>[5x]MSNFKVRDPVIQERLDHDYAHHPLVARMNTLDQGNMSQAEYLVQKRHYLVFLIAHHYYEAYLRRMGGIQRRDHLQTLRDQKPRERADRVSAASAYDAGTFTVPSRPGPASGTTPGGQDSLGVSGSSITTLSSGPHSLSPASDILTTLSSTTETAAPAVADARKPPSGKKK;>[5x]MEATLEQRPFPYLATEANLLTQIKESAADGLFKSFQLLLGKDAREGSVRFEALLGVYTNVVEFVKFLETALAAACVNTEFKDLRRMIDGKIQFKISMPTIAHGDGRRPNKQRQYIVMKACNKHHIGAEIELAAADIELLFAEKETPLDFTEYAGAIKTITSALQFGMDALERGLVDTVLAVKLRHAPPVFILKTLGDPVYSERGLKKAVKSDMVSMFKAHLIEHSFFLDKAELMTRGKQYVLTMLSDMLAAVCEDTVFKGVSTYTTASGQQVAGVLETTDSVMRRLMNLLGQVESAMSGPAAYASYVVRGANLVTAVSYGRAMRNFEQFMARIVDHPNALPSVEGDKAALADGHDEIQRTRIAASLVKIGDKFVAIESLQRMYNETQFPCPLNRRIQYTYFFPVGLHLPVPRYSTSVSVRGVESPAIQSTETWVVNKNNVPLCFGYQNALKSICHPRMHNPTQSAQALNQAFPDPDGGHGYGLRYEQTPNMNLFRTFHQYYMGKNVAFVPDVAQKALVTTEDLLHPTSHRLLRLEVHPFFDFFVHPCPGARGSYRATHRTMVGNIPQPLAPREFQESRGAQFDAVTNMTHVIDQLTIDVIQETAFDPAYPLFCYVIEAMIHGQEEKFVMNMPLIALVIQTYWVNSGKLAFVNSYHMVRFICTHMGNGSIPKEAHGHYRKILGELIALEQALLKLAGHETVGRTPITHLVSALLDPHLLPPFAYHDVFTDLMQKSSRQPIIKIGDQNYDNPQNRATFINLRGRMEDLVNNLVNIYQTRVNEDHDERHVLDVAPLDENDYNPVLEKLFYYVLMPVCSNGHMCGMGVDYQNVALTLTYNGPVFADVVNAQDDILLHLENGTLKDILQAGDIRPTVDMIRVLCTSFLTCPFVTQAARVITKRDPAQSFATHEYGKDVAQTVLVNGFGAFAVADRSREAAETMFYPVPFNKLYADPLVAATLHPLLANYVTRLPNQRNAVVFNVPSNLMAEYEEWHKSPVAAYAASCQATPGAISAMVSMHQKLSAPSFICQAKHRMHPGFAMTVVRTDEVLAEHILYCSRASTSMFVGLPSVVRREVRSDAVTFEITHEIASLHTALGYSSVIAPAHVAAITTDMGVHCQDLFMIFPGDAYQDRQLHDYIKMKAGVQTGPPGNRMDHVGYAAGVPRCENLPGLSHGQLATCEIIPTPVTSDVAYFQTPSNPRGRAACVVSCDAYSNESAERLLYDHSIPDPAYECRSTNNPWASQRGSLGDVLYNITFRQTALPGMYSPCRQFFHKEDIMRYNRGLYTLVNEYSARLAGAPATSTTDLQYVVVNGTDVFLDQPCHMLQEAYPTLAASHRVMLDEYMSNKQTHAPVHMGQYLIEEVAPMKRLLKLGNKVVY;>[2x]MKVQAENAARLGRQVLGLLPPPTHRVSLTRGPEFARGVRDLLSKYAASTRPTVGSLHEALRQAPFRQPTYGDFLVYSQTFSPQEPLGTFLFSFKQEDNGSSMDMLLTPTSLFMLSGMEAAKAPQTHKVAGVWYGSGSGLADFIPNLSELMDTGEFHTLLTPVGPMVQSVHSTFVTKVTSAMKGVGLARDEPRAHVGLTLPCDMLVDLDESCPMVQRREPAGLNVTIYASLVYLRVNQRPSMALTFFQSGKGFAEVVAMIKDHFTDVIRTKYIQLRHELYINRLVFGAVCTLGTVPFDSHPVHQSLNVKGTSLPVLVFANFEAACGPWTVFL;>[4x]MALDKSIVVNLTSRLFADELAALQSKIGSVLPLGDCHRLQNIQALGLGCVCSRETSPDYIQIMQYLSKCTLAVLEEVRPDSLRLTRMDPSDNLQIKNVYAPFFQWDSNTQLAVLPPLFSRKDSTIVLESNGFDIVFPMVVPQQLGHAILQQLLVYHIYSKISAGAPGDVNMAELDLYTTNVSFMGRTYRLDVDNTDPRTALRVLDDLSMYLCILSALVPRGCLRLLTALVRHDRHPLTEVFEGVVPDEVTRIDLDQLSVPDDITRMRVMFSYLQSLSSIFNLGPRLHVYAYSAETLAASCWYSPR;> MDAHAINERYVGPRCHRLAHVVLPRTFLLHHAIPLEPEIIFSTYTRFSRSPGSSRRLVVCGKRVLPGEENQLASSPSGLALSLPLFSHDGNFHPFDISVLRISCPGSNLSLTVRFLYLSLVVAMGAGRNNARSPTVDGVSPPEGAVAHPLEELQRLARATPDPAPTRGPLQVLTGLLRAGSDGDRATHHMALEAPGTVRGESLDPPVSQKGPARTRHRPPPVRLSFNPVNADVPATWRDATNVYSGAPYYVCVYERGGRQEDDWLPIPLSFPEEPVPPPPSLVFMDDLFINTKQCDFVDTLEAACRTQGYTLRQRVPVAIPRDAEIADAVKSHFLEACLVLRGLASEASAWIRAATSPPLGRHACWMDVLGLWESRPHTLGLELRGVNCGGTDGDWLEILKQPDVQKTVSGSLVACVIVTPALEAWLVLPGGFAIKGRYRASKEDLVFIRGRYG;>MLTSERSYLRYPKNRRWTEAGRFWAPHPENVLFIHKPTMEETRRVALGLRSQLVRNRERKTKAHLLSLELDRLVQVHDSRVRVINADIDAVKQMIGNMTWSDNIDMPQSRSHEPPLVTSPPQASHRNFTVAIVPGDPHFSVDRDLRGELMPTLYMNQNQWLPSFGPWFISLTDNAMQRRVFPKELKGTVNFQNSTSLKLISHTLTTVASTTADFFADARHLTDTQAALCLVNAYFCQKTSRQLPATPDDLLADLPQKLDLLITQLKQESGPGDFSFTYSNPQERASLAPLNKESRYPTAFFQRHKLHAMMAKAGLFPHNKGTGAPGTAPAMDLVFAITSAMFGSDIPPFSAYQWNLRAGIVALEVFILAYGLLEFGQVARGHPNRRLNLVSLLGPKFQPGALPDPNAPMLKRGQLFSFISEHYIIPTLQANPNAPVSFIFPGIILAALEARSTVSHKQPGPFVNLTGSRFNEIFEILNQQLTFRDPLALLQARTALRLATEEGLDVLLSHPSPPTLLQEIIKSQFGGGDDYDRAYFMVLGCLPVVLAVV[2x];>MAAQPLYMEGMASTHQANCIFGEHAGSQCLSNCVMYLASSYYNSETPLVDRASLDDVLEQGMRLDLLLRKSGMLGFRQYAQLHHIPGFLRTDDWATKIFQSPEFYGLIGQDAAIREPFIESLRSVLSRNYAGTVQYLIIICQSKAGAIVVKDKTYYMFDPHCIPNIPNSPAHVIKTNDVGVLLPYIATHDTEYTGCFLYFIPHDYISPEHYIANHYRTIVFEELHGPRMDISRGVESCSITEITSPSVSPAPSEAPLRRDSTQSQDETRPRRPRVVIPPYDPTDRPRPPHQDRPPEQAAGYGGNKGRGGNKGRGGKTGRGGNEGRGGHQPPDEHQPPHITAEHMDQSDGQGADGDMDSTPANGETSVTETPGPEPNPPARPDREPPPTPPATPGATALLSDLTATRGQKRKFSSLKESYPIDSPPSDDDDVSQPSQQTAPDTEDIWIDDPLTPLYPLTDTPSFDITADVTPDNTHPEKAADGDFTNKTTSTDADRYASASQESLGTLVSPYDFTNLDTLLAELGRLGTAQPIPVIVDRLTSRPFREASALQAMDRILTHVVLEYGLVSG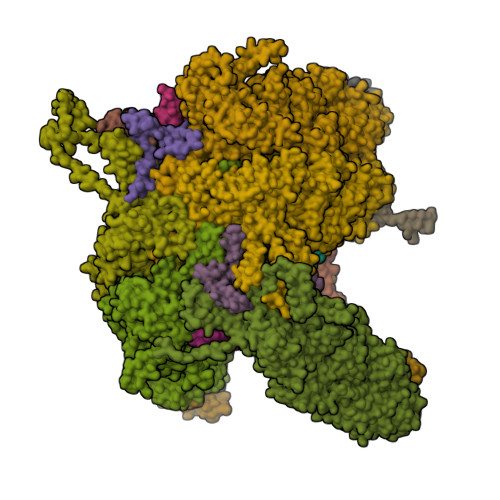YSTAAPSKCTHVLQFFILWGEKLGIPTEDAKTLLESALEIPAMCEIVQQGRLKEPTFSRHIISKLNPCLESLHATSRQDFKSLIQAFNAEGIRIASRERETSMAELIETITARLKPNFNIVCARQDAQTIQDGVGLLRAEVNKRNAQIAQEAAYFENIITALSTFQPPPQSQQTFEVLPDLKLRTLVEHLTLVEAQVTTQTVESLQAYLQSAATAEHHLTNVPNVHSILSNISNTLKVIDYVIPKFIINTDTLAPYKQQFSYLGGELASMFSLDWPHAPAEAVEPLPVLTSLRGKIAEALTRQENKNAVDQILTDAEGLLKNITDPNGAHFHAQAVSIPVLENYVHNAGVLLKGEKSERFSRLKTAIQNLVSSESFITVTLHSTNLGNLVTNVPKLGEAFTGGPHLLTSPSVRQSLSTLCTTLLRDALDALEKKDPALLGEGTTLALETLLGYGSVQDYKETVQIISSLVGIQKLVRDQGADKWATAVTRLTDLKSTLATTAIETATKRKLYRLIQRDLKEAQKHETNRAMEEWKQKVLALDNASPERVATLLQQAPTAKAREFAEKHFKILLPVPADAPVQASPTPMEYSASPLPDPKDIDRATSIHGEQAWKKIQQAFKDFNFAVLRPADWDALAAEYQRRGSPLPAAVGPALSGFLETILGTLNDIYMDKLRSFLPDAQPFQAPPFDWLTPYQDQVSFFLRTIGLPLVRALADKISVQALRLSHALQSGDLQQATVGTPLELPATEYARIASNMKSVFNDHGLQVRSEVADYVEAQRADAHTPHVPRPKIQAPKTLIPHPDAIVADGLPAFLKTSLLQQEAKLLALQRADFESLESDMRAAEAQRKASREETQRKMAHAITQLLQQAPSAISGRPLSLQDPVGFLEGIIYDKVLERESYETGLEGLSWLEQTIKSITVYAPVEEKQRMHVLLDEVKKQRANTETALELEAAATHGDDARLLQRAVDELSPLRVKGGKAAVESWRQKIQTLKSLVQEAEQAGLLLATIDTVAGQAQETISPSTLQGLYQQGQEAMAAIKRFRDSPQLAGLQEKLAELQQYVKYKKQYLEHFEATQSVVFTAFPLTQEVTIPALHYAGPFDNLERLSRYLHIGQTQPAPGQWLLTLPTFDPTRPACVPAGGHEPPLHRQVVFSSFLEAQIRLALSVAGPVPGRGLPGTPQIRRGVEAAACFLHQWDEISRLLPEVLDTFFHNAPLPAESSSNAFLAMCVLTHLVYLAGRAVLGPREPEHAAPDAYPREVALAPRDLTYLLLAMWPSWISAILKQPSHAEAAHACLVTLPTMLKAVPYLTLEASAGPLPADMRHFATPEARLFFPARWHHVNVQEKLWLRNDFMSLCHRSPGRARIAVLVWAVTCLDPEVIRQLWSTLRPLTADESDTASGLLRVLVEMEFGPPPKTPRREAVAPGATLPPYPYGLATGERLVGQAQERSGGAGKMPVSGFEIVLGALLFRAPLRIFSTASTHRISDFEGGFQILTPLLDCCPDREPFASLAAAPRRTVPLGDPCANIHTPEEIQIFARQAAWLQYTFANYQIPSTDNPIPIVVLNANNNLENSYIPRDRKADPLRPFYVVPLKPQGRWPEIMTTATTPCRLPTSPEEAGSQFARLLQSQVSATWSDIFSRVPERLAPNATQKSSQTMSEIHEVAATPPLTITPNKPTGTPHVSPEADPITERKRGQQPKIVADNMPSRILPSLPTPKPREPRITLPHALPVISPPAHRPSPIPHLPAPQVTEPKGVLQSKRGTLVLRPAAVIDPRKPVSAPITRYERTALQPPRTEGEGRRPPDTQPVTLTFRLPPTAPTPATAALETKTTPPSTPPHAIDISPPQTPPMSTSPHARDTSPPAEKRAAPVIRVMAPTQPSGEARVKRVEIEQGLSTRNEAPPLERSNHAVPAVTPRRTVAREIRIPPEIKAGWDTAPDIPLPHSSPESSPPTSPQPIRVDDKSPLPNLVERYARGFLDTPSVEVMSLENQDIAVDPGLLTRRIPSVVPMPHPIMWSPIVPISLQNTDIDTAKITLISFIRRIKQKVAALSASLAETVDRIKKWYL[2x]> RRNVEARGIRRSPVVTPDIQIGHGEDAIEMDLYRYLLSNRIIFIGGYINDKMATQIVGSLMALE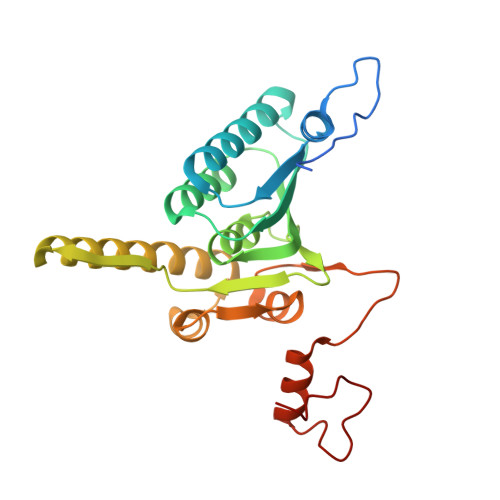AVDENEDIRIYINSPGGQPYSVLGVVDAMQSIKPDVQTVALGACYSYASLVVAAGTKGKRYAMKNTRLMMTQPMGGSQGDIYQIKATVEELNALYQIFSRYYMKFTGMNQDQIEQATCRDHFMTPEQAKLEGLIDEIIRGKGDYTVPPAIVRQFREVGLVDDLTPGPFLKVDCN10-PARPARGYL-5,8-DIDEAZAFOLATE-4-GLUTAMIC ACID | C39 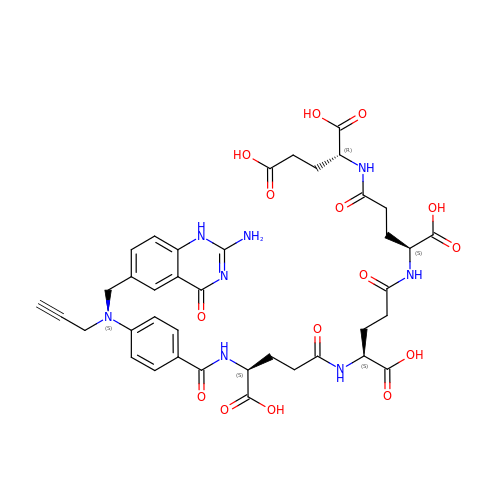H44 N8 O15 | SASAWWASHFSVQE-QGMKSFRFSA-N>[2x]MAWPKVQPEVNIGVVGHVDHGKTTLVQAITGIWTSKHSEELKRGMTIKLGYAETNIGVCESCKKPEAYVTEPSCKSCGSDDEPKFLRRISFIDAPGHEVLMATM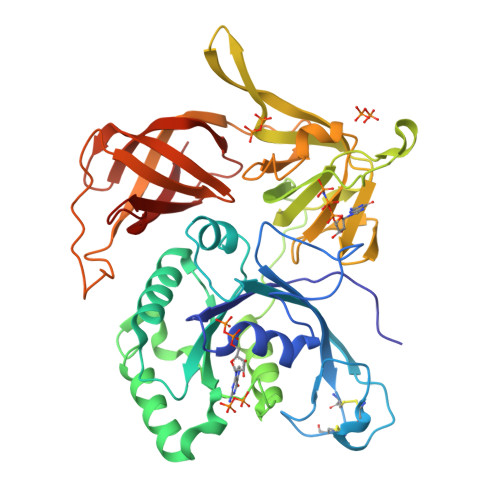LSGAALMDGAILVVAANEPFPQPQTREHFVALGIIGVKNLIIVQNKVDVVSKEEALSQYRQIKQFTKGTWAENVPIIPVSALHKINIDSLIEGIEEYIKTPYRDLSQKPVMLVIRSFDVNKPGTQFNELKGGVIGGSIIQGLFKVDQEIKVLPGLRVEKQGKVSYEPIFTKISSIRFGDEEFKEAKPGGLVAIGTYLDPSLTKADNLLGSIITLADAEVPVLWNIRIKYNLLERVVGAKEMLKVDPIRAKETLMLSVGSSTTLGIVTSVKKDEIEVELRRPVAVWSNNIRTVISRQIAGRWRMIGWGLVEI> GAMAKKLSRTISGVTPVAVMTKPLPCPGKCIYCPTFAATPQSYTPESPAVLRAKSCEYQAYKQVALRLRIIQDMGHPTDKVELIIMGGTFLSADITYQYGFIKDCYDALNGVVAGSLEEAKTINETAQHRCVGLCIETRPDICGKAEIQRMIDFGTTRVELGVQMLDDDIYKLVERGHRVSDVAEATCLLREYGLKVHYHWMPGLPGSSPEKDLALSRMVFEDPRFCPDGLKLYPTMVVEGTILEQWWKEGRYTPYPNGTMTGLIADIKALVPPYVRISRVLRDIPAVFISAGLKDSLRDGVRQILESRHQKCRCIRCREYGHRQRKGQTSGEPTLRRLDYPASGGKEIFLSFEDASDTLYGLLRLRIPCASLPVLGQKYGAKTGLVRALHVGSGSGRGLGRKLLAEAECLARDEFGLDSLAILSGVGAREYYRSLGYELVAGYMCKHLD

Elp3 acts as the catalytic subunit, but the loss of any of the six subunits results in hypo-modified U34 tRNAs in yeast, indicating that the complete integrity of the complex is important for its function. The enzymatically active Elp3 subunit of Elongator contains two functional domains, utilizes multiple cofactors, and conducts a unique uridine base modification specifically found only at the wobble base position of tRNAs. The two domains form a cleft that contains several highly conserved basic residues, which bind and accommodate the tRNA anticodon stem loop (ASL). The current model of a radical based Elp3-mediated cm5-modification reaction is proposed as follows (i) Elp3 recruits SAM and cleaves it to generate a 5’deoxyadenosine radical (5’-dA) in the rSAM domain, (ii) Elp3 hydrolyzes acetyl-CoA in the KAT domain and (iii) an acetyl radical is formed by the products of the two domains and (iv) is transferred onto the C5 position of U34 in the bound tRNA molecule.

To obtain detailed structural insights into acetyl-CoA coordination, we combined the respective blocking loop deletion (DmcElp3390–406(GSGSG)) with additional active site mutations (e.g. E386A, H388A, R411T) for co-crystallization trials in the presence of acetyl-CoA and different acetyl-CoA analogues. We successfully co-crystallized DmcElp3390–406(GSGSG)/E386A in complex with desulfo-CoA (DmcElp3-DCA) using similar crystallization conditions as for apo DmcElp3. The overall structure of DmcElp3-DCA closely matches the structure of DmcElp3, indicating that ligand binding has very little or no influence on the structural arrangement of the two domains or the Fe–S cluster mediated rSAM dimerization. DCA is structurally similar to acetyl-CoA but lacks both, the acetyl group as well as the thiol-moiety, and therefore represents a post-cleavage product analogue. DCA binds to the KAT domain of DmcElp3 in a similar way as acetyl-CoA is coordinated by the active site of GCN5 from Tetrahymena. In detail, the two phosphate groups of DCA are in close proximity to the glycine residues residing at the start of the blocking loop. The rest of DCA, including pantothenic acid and β-mercaptoethylamine, are pointing deeper into the predicted binding pocket. Furthermore, previously identified conserved residues, including K77, K193, and Y441, are involved in ligand binding and in close proximity to DCA. The β-mercaptoethylamine part of DCA was not clearly resolved in our densities, presumably because this part of the ligand is flexible in the absence of the missing tRNA substrate. Considering the observation that DCA stays bound even in the absence of the transferable acetyl group, we conclude that the cleavage products stay associated with the KAT domain until the next round of modification is initiated.> PGYTFTSITLKPPKIDRGSYYGKRLLLPDSVTEYDKKLVSRLQIRVNPLPKFDSTVWVTVRKVPASSDLSVAAISAMFADGASPVLVYQYAASGVQANNKLLYDLSA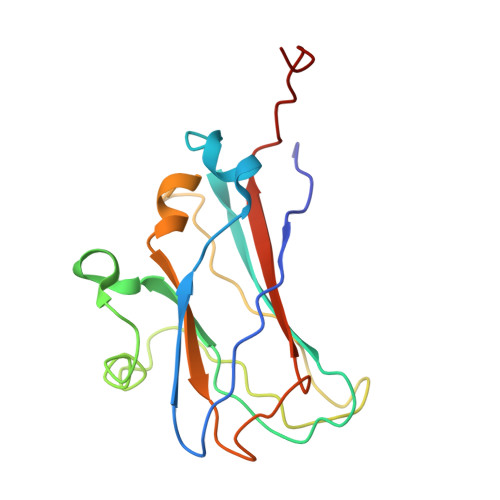MRADIGDMRKYAVLVYSKDDALETDELVLHVDIEHQRIPTSGVLPV>MGHHHHHHKLNTDNPIYAYIVGLFEGDGWITISKKGKYLLYELGIEMHIRDIQLLYKIKNILGIGKVTIKKLKMKDGTIKEMCKFNVRNKNHLKNIIIPIFNKYPMLTNKHYDYLYFKDN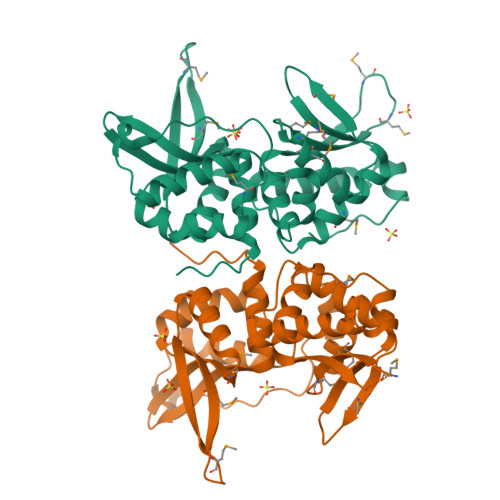LLKDIKYYNDLSYYLRPIKPFNTTEDILNKNYFSSWLIGFFEAKSCFSIYKPMNKKMKTASFEVSMNNNMEVMLAIKSYLKINNNIYMNEFNNSKMTTKSINDIKNVVMFINNNPIKLLGYKKLQYLLFLKDLRTITKYNNYFKIPSKY[2x]>HHHHHHSSGLEVLFQGPMSDNTLSQKENMYPEINIKAMNQAVNTIWLLAQRQTSGIEIINDKVKRISLYSREFDEMMRDSLAQLAPVLKQLTSDAAFQTIAQIDEALADPSLSKDDREALTLERNNLIQNLSKHIDNVIVSFTGRTSKLTNKISDISDMVIAERLQDLVTQTESQKTELQSDIDPKTEKRNKLDADREKIIESQDVIRQNNIADMFKDFIPSAKDIDGLDFTQPKKEAIKQAIKQGAEIARKILGKVSEGLKYIDLADARMKLSDQIDQLITETDELKAKIREVELRLSGLKDVMQIDTERTTLLTEAVKIEQVWISFAEQLHKLSNDEINQQDLSNLINGQLDFLNNLTLQYNKLK[4x]

α-Xenorhabdolysin is a PFT that has been first isolated from the bacterium Xenorhabdus nematophila. Xenorhabdolysins are also found in other entomopathogenic bacteria, such as Photorhabdus luminescens, and human pathogenic bacteria, such as Yersinia enterocolitica and Proteus mirabilis. They are composed of two subunits, namely XaxA (45 kDa) and XaxB (40 kDa) and are only active when the two components act together. Xenorhabdolysins, which were suggested to be binary toxins, perforate the membranes of erythrocytes, insect granulocytes and phagocytes and induce apoptosis. In contrast to previous predictions, XaxAB is therefore not a typical binary toxin, but rather a bi-component α-PFT.

XaxB also crystallized in orthorhombic space group P212121 with a unit cell dimension of 89 × 99 × 194 Å and four molecules per AU. The diffraction data of XaxB was processed with the XDS package and SeMet atoms were determined using the CRANK2 pipeline in the CCP4 software package. The four XaxB molecules in the asymmetric unit differ considerably in their tail domain. Especially, helices αB and αC that protrude slightly from the five-helix-bundle take different positions. Although this might be due to tight crystal packing, it also indicates a certain degree of flexibility of the tail domain of XaxB. In contrast to XaxA the head domain of XaxB contains in addition to the central coiled-coil a helix-loop-helix motif, dividing helix αE and a 21-residue long amphipathic helix (αF). The highly conserved hydrophobic face of helix αF is oriented toward helices αD and αG and thereby shielded from the solvent. The conformation of the head domain is stabilized by conserved hydrophobic as well as electrostatic interactions, including putative salt bridges. Interestingly, in the case of XaxB the tongue is formed by an amphipathic helix, while XaxA does not contain such motif. We identified two hinge regions that facilitate the swinging out movement of αF in XaxB.>MPQTAGPDTIRILVSTDNHVGYEERDPIRKDDSWRTFDEIMQLARTKDVDMVLLGGDLFHDNKPSRKAMYQVMRSLRKNCLGMKPCELEFLSDPAEVFEGAFPHVNYYDPDINVSIPVFSIHGNHDDPSGDGHLCSLDLLQVAGLVNYFGRVPEADNIHVKPILLQKGKTKLALYGMSNVRDERIHRTFRDNKVRFYRPSQQTGDWFNLLTLHQ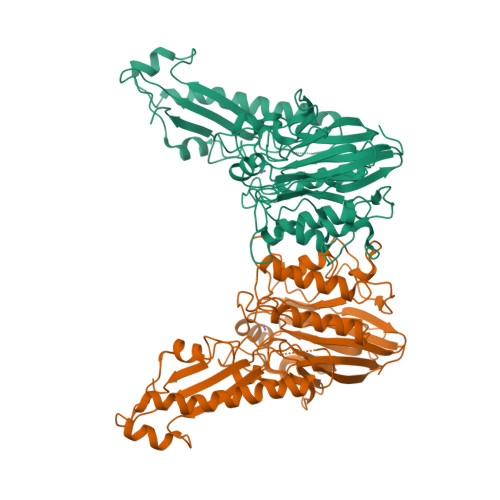NHYAHTPTGYLSENMLPDFLDLVIWGHEHECLIDPKKNPETGFHVMQPGSSIATSLVPGEAVPKHIAILSITGKSFEVEKIPLRTVRPFVIREITLATDKRFKGLEKKQDNRQEVTKRLMQIVEEMIAEANEMWRSLHEDSQDDEDEEQPLPLIRLKVEYSSPEGTKFEVENPQRFSNRFAGKVANQNDVVHFYRKKTGTTRKPKEGKRELPEGIAEALEDSDSISVDALVQEFFAQQSLKILPQAPFGDAVNQFVSKDDKHAVEMFVMDSLSSQVRGLLQLDDDKINEGLDSHIEDFRKVMEKNFLSGQQKQAQRRRRFKEKAAALEHHHHHH[2x]N-{8-[(8-{[(E)-AMINO(IMINO)METHYL]AMINO}OCTYL)AMINO]OCTYL}GUANIDINE 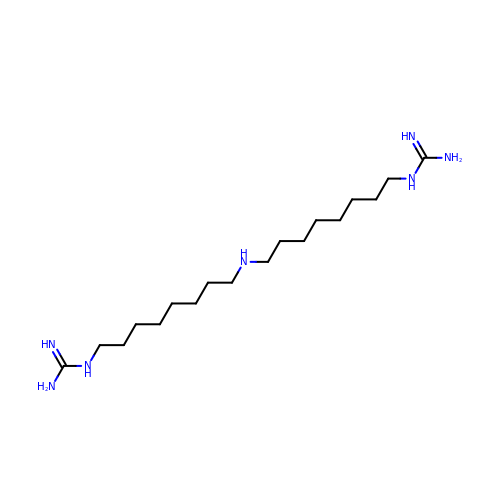| C18 H41 N7 | RONFGUROBZGJKP-UHFFFAOYSA-N>[2x]GTGAESTAERSARFERDALEFLDQMYSAALRMTRNPADAED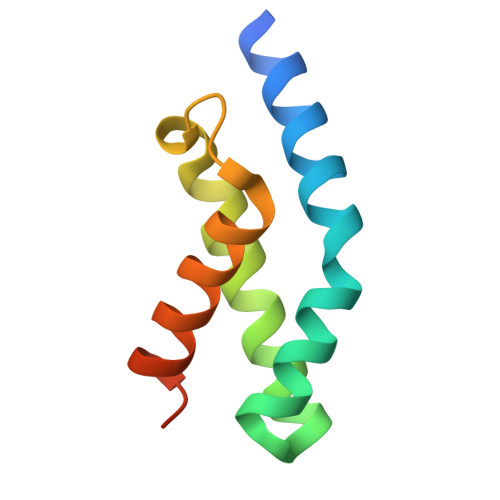LVQETYAKAYASFHQFREGTNLKAWLYRILTNTFINSYRKKQREPQ> MALVYDAEFVGSEREFEEERETFLKGVKAYDGVLATRYLMERSSSAKNDEELLELHQNFILLTGSYACSIDPTEDRYQNVIVRGVNFDERVQRLSTGGSPARYAIVYRRGWRAIAKALDIDEEDVPAIEVRAVKRNPLQPALYRILVRYGRVDLMPVTVDEVPPEMAGEFERLIERYDVPIDEKEERILEILRENPWTPHDEIARRLGLSVSEVEGEKDPESSGIYSLWSRVVVNIEYDERTAKRHVKRRDRLLEELYEHLEELSERYLRHPLTRRWIVEHKRDIMRRYLEQRIVECALKLQDRYGIREDVALCLARAFDGSISMIATTPYRTLKDVCPDLTLEEAKSVNRTLATLIDEHGLSPDAADELIEHFESIAGILATDLEEIERMYEEGRLSEEAYRAAVEIQLAELTKKEGVGRKTAERLLRAFGNPERVKQLAREFEIEKLASVEGVGERVLRSLVPGYASLISIRGIDRERAERLLKKYGGYSKVREAGVEELREDGLTDAQIRELKGLKTLESIVGDLEKADELKRKYGSASAVRRLPVEELRELGFSDDEIAEIKGIPKKLREAFDLETAAELYERYGSLKEIGRRLSYDDLLELGATPKAAAEIKGPEFKFLLNIEGVGPKLAERILEAVDYDLERLASLNPEELAEKVEGLGEELAERVVYAARERVESRRKSGRQERSEEEWKEWLERKVGEGRARRLIEYFGSAGEVGKLVENAEVSKLLEVPGIGDEAVARLVPGYKTLRDAGLTPAEAERVLKRYGSVSKVQEGATPDELRELGLGDAKIARILGLRSLVNKRLDV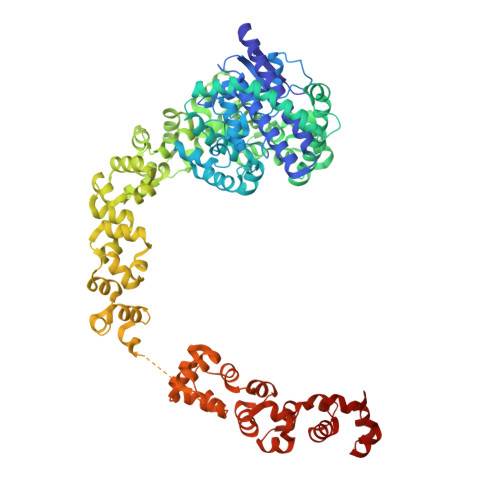DTAYELKRRYGSVSAVRKAPVKELRELGLSDRKIARIKGIP>XRMKQIEDKIEEIESKQK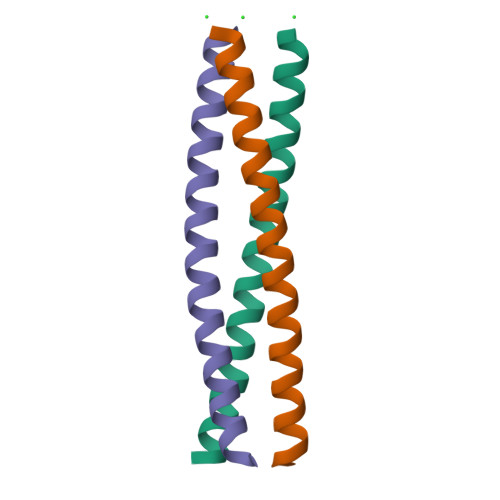KIENEIARIKKLLQLTVWGIKQLQARIL[3x]> GPHMGAKWHLGIRSQSKPNDIMLE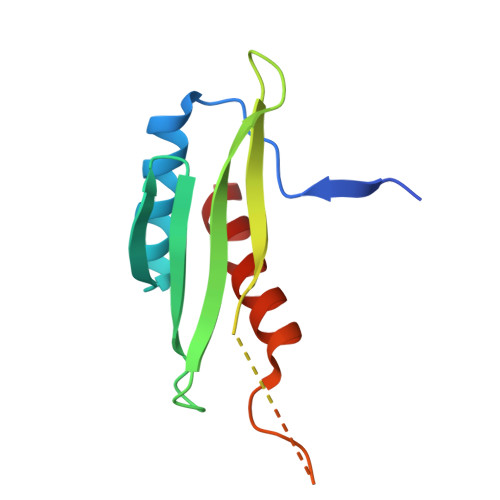VYRAMKALSYEWKIINPYHVRVRRQNVKTGKFSKMSLQLYQVDAKSYLLDFKSLTNDEVEQGDDVIMESLTPPPLSVSGVMPLQPTGHHTMEFFEMCAALIIQLAR>[2x]KLGKLQYSLDYDFQNNQLLVGIIQAAELPALDMGGTSDPYVKVFLLPDKKKKFETKVHRKTLNPVFNEQFTFKVPYSELGGKTLVMAVYDFDRFSKHDIIGEFKVPMNTVDFGHVTEEWRDLQSAEK;>[4x]KLGKLQYSLDYDFQNNQLLVGIIQAAELPALDMGGTSDPYVKVFLLPDKKKKFETKVHRKTLNPVFNEQFTFKVPYSELGGKTLVMAVYDFDRFSKHDIIGEFKVPMNTVDFGHVTEEWRDLQSAEKEEQEKLGDICFSLRYVPTAGKLTVVILEAKNLKKMDVGGLSDPYVKIHLMQNGKRLKKKKTTIKKNTLNPYYNESFSFEVPFEQIQKVQVVVTVLDYDKIGKNDAIGKVFVGYNSTGAELRHWSDMLANPRRPIAQWHTLQVEEEVDAMLAVKK;>GSNR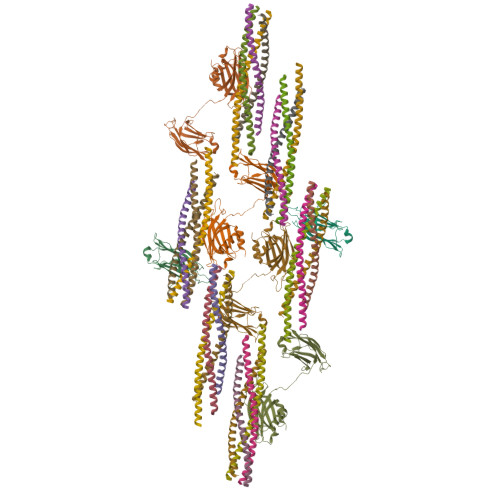RLQQTQAQVDEVVDIMRVNVDKVLERDQKLSELDDRADALQAGASQFETSAAKLKRKYW[6x];>MALSEIETRHSEIIKLENSIRELHDMFMDMAMLVESQGEMIDRIEYNVEHAVDYVERAVSDTKKAVK[6x];>[6x]MRNELEEMQRRADQLADESLESTRRMLQLVEESKDAGIRTLVMLDEQGEQLDRVEEGMNHINQDMKEAEKNLKDLGK;>[6x]MARENEMDENLEQVSGIIGNLRHMALDMGNEIDTQNRQIDRIMEKADSNKTRIDEANQRATKMLG> NTIQQLMMILNSASDQPSENLISYFNNCTVNPKESILKRVKDIGYIFKEKFAKAVGQGCVEIGSQRYKLGVRLYYRVMESMLKSEEERLSIQNFSKLLNDNIFHMSLLACALEVVMATYSRSTSQNLDSGTD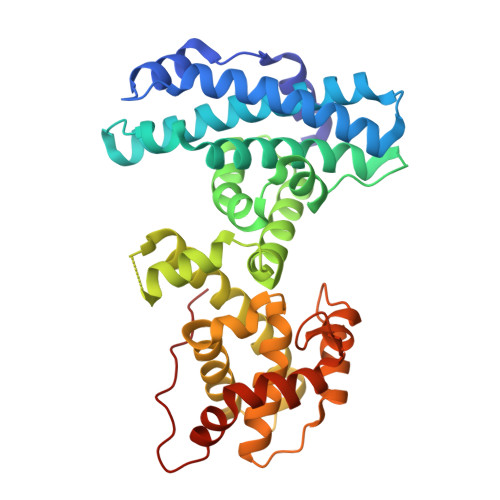LSFPWILNVLNLKAFDFYKVIESFIKAEGNLTREMIKHLERCEHRIMESLAWLSDSPLFDLIKQSKDREGKSTSLSLFYKKVYRLAYLRLNTLCERLLSEHPELEHIIWTLFQHTLQNEYELMRDRHLDQIMMCSMYGICKVKNIDLKFKIIVTAYKDLPHAVQETFKRVLIKEEEYDSIIVFYNSVFMQRLKTNILQYASTRPPTLSPIPHIPR>GEPRTKRQAISAEPTAFDIQDLSHVTLPFYPKSPQSKDLIKEAILDNDFMKNLELSQIQEIVDCMYPVEYGKDSCIIKEGDVGSLVYVMEDGKVEVTKEGVKLCTMGPGKVFGELAILYNCTRTATVKTLVNVKLWAIDRQCFQTIMMRTGLIKHTEYMEFLKSVPTFQSLPEEILSKLADVLEETHYENGEYIIRQGARGDTFFIISKGTVNVTREDSPSEDPVFLRTLGKGDWFGEKALQGEDVRTANVIAAEAVTCLVIDRDSFKHLIGGLDDVSNKAYEDAEAKAKYEAEAAFFANLKLSDFNIIDTLGVGGFGRVELVQLKSEESKTFAMKILKKRHIVDTRQQEHIRSEKQIMQGAHSDFIVRLYRTFKDSKYLYMLMEACLGGELWTILRDRGSFEDSTTRFYTACVVEAFAYLHSKGIIYRDLKPENLILDHRGYAKLVDFGFAKKIGFGKKTWTFCGTPEYVAPEIILNKGHDISADYWSLGILMYELLTGSPPFSGPDPMKTYNIILRGIDMIEFPKKIAKNAANLIKKLCRDNPSERLGNLKNGVKDIQKHKWFEGFNWEGLRKGTLTPPIIPSVASPTDTSNFDSFPEDNDEPPPDDNSGWDIDF[2x]

Cyclic GMP-dependent protein kinases (PKGs) are key mediators of the nitric oxide/cyclic guanosine monophosphate (cGMP) signaling pathway that regulates biological functions as diverse as smooth muscle contraction, cardiac function, and axon guidance. PKGs belong to the AGC family of protein kinases and have N-terminal regulatory (R) and C-terminal catalytic (C) domains. The R-domain comprises a leucine zipper (LZ) domain, a linker region with an auto-inhibitory (AI) sequence, and two cyclic nucleotide-binding (CNB-A and -B) domains. By analogy to PKA, the PKG R-domain is thought to bind via its AI sequence to the C-domain active site to form an auto-inhibited R:C state; binding of cGMP to the R-domain destabilizes this state and allows active kinase to phosphorylate downstream substrates.

Here, we present the first crystal structure of PKG Iβ in which the regulatory domain is free of cyclic nucleotide and adopts an AI state bound to the catalytic domain. In the PKG Iβ 71–686 AI complex, the two CNB domains contact the large lobe of the C-domain while the AI sequence docks to the C-domain active site. The C-domain binds AMP-PNP:Mn2+ at the ATP site with the DFG motif adopting an ‘in’ conformation. Both CNB-A and CNB-B PBCs adopt ‘open’ conformations with respect to the β-subdomains, similar to previous CNB domain structures without cyclic nucleotide. In the R:C complex we present here, the interdomain linker between the tandem CNB domains forms a single helix that allows the two CNB domains to clamp around the C-domain. The overall structure is very similar to the PKA RIα:Cα heterodimer showing square root of the average of squared errors (RMSD) values of 1.95 Å for 546 shared Cα atoms, and it is similar to the CNB-A/B and the catalytic domains of monomeric Plasmodium PKG showing RMSD values of 2.91 Å for 504 shared Cα atoms. The R:C interface reveals specific contacts between the PKG Iβ AI sequence and the active site that help to explain isoform-specific activation constants and the activating effects of phosphorylation in the linker. In the AI PKG Iβ C-domain, the glycine-rich loop contacts bound AMP-PNP, activation loop T532 is phosphorylated, and the DFG motif adopts an ‘in’ conformation with D517 coordinating Mn2+, so the pseudo-substrate is bound much as true substrates are expected to bind for phosphorylation. CNB-A in the auto-inhibited PKG Iβ holoenzyme adopts an ‘open’ PBC conformation typical of apo CNBs, and its contacts with the C-domain indicate that the orientation of the PBC is critical to auto-inhibition.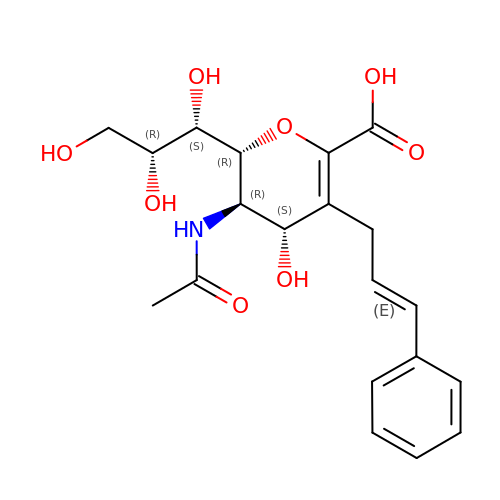5-acetamido-2,6-anhydro-3,5-dideoxy-3-[(2E)-3-phenylprop-2-en-1-yl]-D-glycero-L-altro-non-2-enonic acid | C20 H25 N O8 | LRXKGKMIXXSWGY-KXNCHKOWSA-N Anti-chemokine activity has been described in the extracts of tick salivary glands, and we have recently described the cloning and characterization of such chemokine binding proteins from a tick salivary gland cDNA library, which we have named Evasins. Evasin-1 is a small 94-amino acid protein which binds CCL3/MIP-1α and CCL4/MIP-1β with very high affinity (0.16 and 0.81 nM, respectively), and also displays lower affinity binding (3.2 nM) to a closely related member of the CC chemokine family, CCL18/ PARC. This chemokine-binding protein does not share any relevant sequence or structural homology to any other known proteins, notably the viral chemokine-binding proteins, and moreover, is considerably smaller, being only 10 kDa compared to the viral proteins which range in size between 30–40 kDa. The Evasin-1 secondary structure is composed of seven beta strands forming three anti-parallel beta sheets, one short alpha helix, and contains four disulfide bridges.

In order to understand the structural basis of the chemokine binding mechanism by Evasin-1, we have crystallized the complex (accession code: 3 fpu) between Evasin-1 and a variant of the human chemokine CCL3. One monomer of Evasin-1 binds one monomer of CCL3 displaying a 1∶1 stoichiometry. Upon complex formation, the N-terminal region of CCL3 interacts with both the N-terminal and C-terminal regions of Evasin-1. The complex formation induces the stabilization of the entire N-terminal and C-terminal areas of Evasin-1 and of the N-terminal segment of CCL3, which becomes visible in the electron density maps, showing the rearrangement of both N-terminal ends upon binding. Due to interactions in the complex, the CCL3 N-terminal region (residues Ser2-Thr10) moves by almost 90 degrees with 5AlaB moving circa 20 Å. Three additional secondary structure elements are formed upon binding: the α2 3-10 helix at the C-terminal of Evasin-1; and the α0 3-10 helix and β0 strand at the N-terminal region of CCL3. Three specific residues of CCL3, Thr16B-Ser17B-Arg18B, are targeted by the N-terminal region of Evasin-1, through 7 hydrogen bonds. The N-terminal contacts include several hydrophobic interactions, one of which is an important edge-to-face π-π interaction between Phe14A from Evasin-1 and Phe13B from CCL3. The C-terminal of Evasin-1 embraces the N-terminal part of CCL3 due to an important network of hydrogen bonds and comprising a very important hydrophobic stacking interaction between the Trp89A from Evasin-1 and Phe29B of CCL3. The crystal structure reveals the C-terminal polyhistidine tag, and includes two metal ions, modelled as Ni2+ atom (believed to be leached from the IMAC resin during purification) and which play an important role in establishing the crystal lattice.

> EDDEDYGDLGGCPFLVAENKTGYPTIVACKQDCNGTTETAPNGTRCFSIGDEGLRRMTANLPYDCPLGQCSNGDCIPKETYEVCYRRNWRDKKNHHHHHH;> MSLAADTPTTCCFSYTSRQIPQNFIADYFETSSQCSKPGVIFLTKRSRQVCADPSEEWVQKYVSDLELSA> AKGSVLVTDAEGQPVADATVEFKVYNYAEFYTVATKHTDRSGHASLTAGKGDMLVWASKDGRFGYSKLSFGKDNE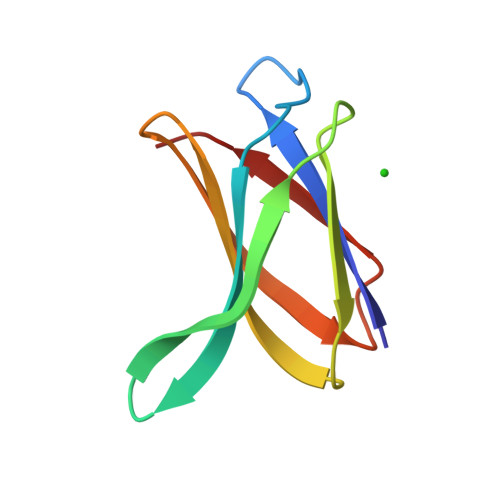LKITLDK>GSECSTQLDIVIVLDGSNSIYPWDSVTAFLNDLLKRMDIGPKQTQVGIVQYGENVTHEFNLNKYSSTEEVLVAAKKIVQRGGRQTMTALGTDTARKEAFTEARGARRGVKKVMVIVTDGESHDNHRLKKVIQDCEDENIQRFSIAILGSYNRGNLSTEKFVEEIKSIASEPTEKHFFNVSDELALVTIVKTLGERIF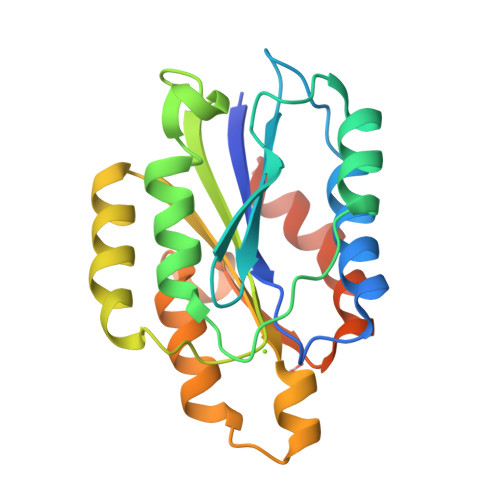ALEATAVDSSGRIVTD[2x]>[2x]MLDIKLIRENPELVKNDLIKRGELEK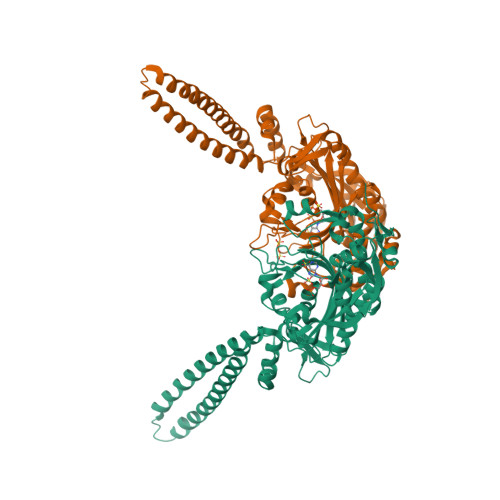VKWVDEILKLDTEWRTKLKEINRLRHERNKIAVEIGKRRKKGEPVDELLAKSREIVKRIGELENEVEELKKKIDYYLWRLPNITHPSVPVGKDENDNVPIRFWGKARVWKGHLERFLEQSQGKMEYEILEWKPKLHVDLLEILGGADFARAAKVSGSRFYYLLNEIVILDLALIRFALDRLIEKGFTPVIPPYMVRRFVEEGSTSFEDFEDVIYKVEDEDLYLIPTAEHPLAGMHANEILDGKDLPLLYVGVSPCFRKEAGTAGKDTKGIFRVHQFHKVEQFVYSRPEESWEWHEKIIRNAEELFQELEIPYRVVNICTGDLGYVAAKKYDIEAWMPGQGKFREVVSASNCTDWQARRLNIRFRDRTDEKPRYVHTLNSTAIATSRAIVAILENHQEEDGTVRIPKVLWKYTGFKEIVPVEKKERCCAT>MADVETETGMIAQWIVFAIMAAAAIAFGVAVHFRPSELKSAYYINIAICTIAATAYYAMAVNYQDLTMNGERQVVYARYIDWVLTTPLLLLDLIVMTKMGGVMISWVIGADIFMIVFGILGAFEDEHKFKWVYFIAGCVMQAVLTYGMYNATWKDDLKKSPEYHSSYVSLLVF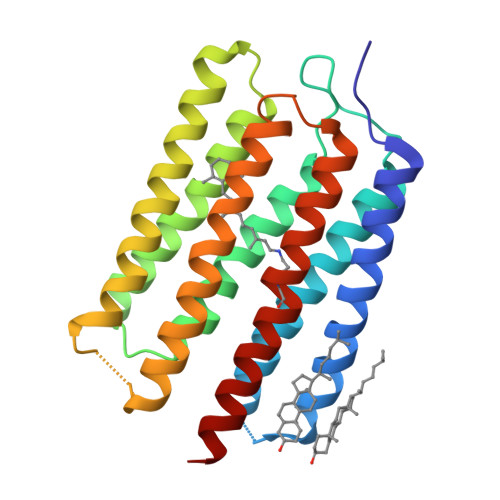LSILWVFYPVVWAFGSGSGVLSVDNEAILMGILDVLAKPLFGMGCLIAHETIFKKM[4x]1,3-dihydroisoindol-2-yl-[(2R,4S)-4-phenylpyrrolidin-1-ium-2-yl]methanone 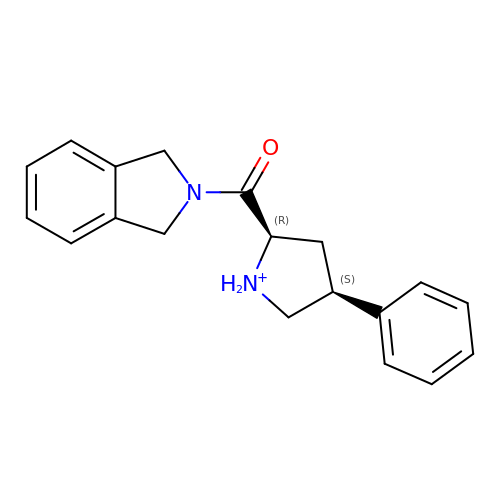| C19 H21 N2 O | CNNYTLGFUDHERQ-QZTJIDSGSA-O> MAETRVIVVGNEKGGAGKSTIAVHLVTALLYGGAKVAVIDLDLRQRTSARFFENRRAWLDNKKIELPEPLALNLSDNDVALAERPEEEQVAGFEAAFARAMAECDFILIDTPGGDSAITRMAHGRADLVVTPMNDSFVDFDMLGTVDPVTLELTKPSLYSLTVWEGRKQRALSGQRQAMDWVVLRNRLATTEARNRKRLEDRLNALAKRVGFRIGPGLRDRVIYRELFPFGLTIADLSPQVRPVPVSLQHLAARQELRALMHSLGLSAYSGETMLAAQGSHHHHHH

Protein gradients play a central role in the spatial organization of cells, but the mechanisms of their formation are incompletely understood. This study analyzes the determinants responsible for establishing bipolar gradients of the ATPase MipZ, a key regulator of division site placement in Caulobacter crescentus. MipZ dynamically interacts with the polar ParB-parS complexes, forming a subcellular gradient with concentration maxima at the tips of the cell and a minimum at the cell center. It inhibits polymerization of the tubulin homolog FtsZ into the so-called Z ring, a structure that forms the basis of the bacterial divison apparatus (Erickson et al., 2010). MipZ belongs to the Mrp/MinD family of P loop ATPases, a heterogeneous group of proteins that act as nucleotide-dependent molecular switches (Leipe et al., 2002).

The two independent structures show excellent agreement with a root-mean-square deviation (rmsd) of 0.44 Å. Superimposition of the structures reveals that MipZ, Soj and MinD share significant similarity in the region constituting the nucleotide-binding site, with an rmsd of 2.4 Å across the 176 α-carbons forming the backbone of the conserved core. However, MipZ differs from its family relatives in the arrangement of several conserved loops. In addition, it displays a number of unique features, including a marked extension of helix 2 and a large loop between helices 9 and 10 (helices 10/11 in Soj). Notably, helices 6 and 7 of MipZ correspond to a single helix in both Soj and MinD (helix 8 in Soj). At the junction of these two helices, MipZ exhibits an unusual structural motif, consisting of a large loop that is stabilized by a short antiparallel β sheet (S6/S7). Together, these distinct characteristics are consistent with a clear evolutionary separation of MipZ from its two relatives. MipZ has no C-terminal amphipathic helix, as used for membrane attachment of MinD, and lacks the conserved DNA-binding domain characteristic of plasmid-encoded ParA proteins (Gerdes et al., 2010). Interaction analyses showed that MipZ monomers bind to ParB irrespective of their nucleotide state. Monomers are unable to interact with the nucleoid and, consequently, display high diffusional mobility, thereby rapidly returning to the polar ParB clusters.> ADGPYLVIVEQPKQRGFRFRYGCEGPSHGGLPGASSEKGRKTYPTVKICNYEGPAKIEVDLVTHSDPPRAHAH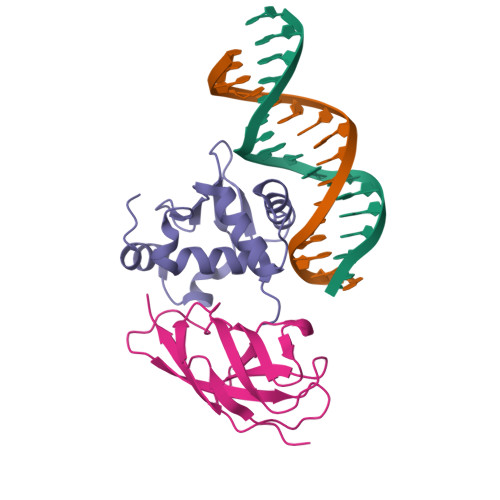SLVGKQCSELGICAVSVGPKDMTAQFNNLGVLHVTKKNMMGTMIQKLQRQRLRSRPQGLTEAEQRELEQEAKELKKVMDLSIVRLRFSAFLRASDGSFSLPLKPVISQPIHDSKSPGASNLKISRMDKTAGSVRGGDEVYLLCDKVQKDDIEVRFYEDDENGWQAFGDFSPTDVHKQYAIVFRTPPYHKMKIERPVTVFLQLKRKRGGDVSDSKQFTYYPLV;> GSGPIQLWQFLLELLTDKSCQSFISWTGDGWEFKLSDPDEVARRWGKRKNKPKMNYEKLSRGLRYYYDKNIIHKTAGKRYVYRFVCDLQSLLGYTPEELHAMLDVKPDADE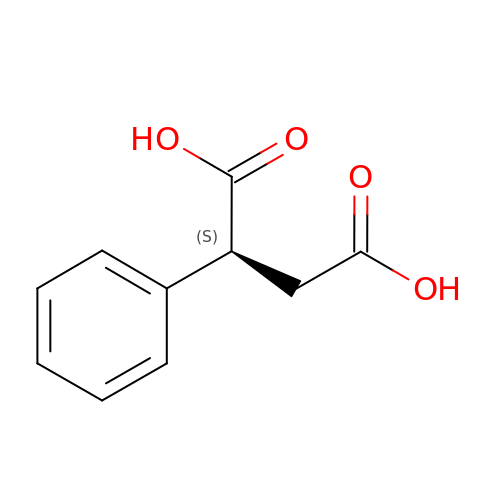(2S)-2-phenylbutanedioic acid | C10 H10 O4 | LVFFZQQWIZURIO-QMMMGPOBSA-N Ral GTPases have been implicated as critical drivers of cell growth and metastasis in numerous Ras-driven cancers. Upon association with and activation by Ras·GTP, RalGDS activates the Ral (Ras-like) small GTPases, RalA, and RalB. The Ral GTPases share a panel of effectors including RLIP76 (also called RalBP1), members of the exocyst complex (Sec5 and Exo84), and the transcription factor ZONAB. Our solution structure of the RBD of RLIP76 in complex with RalB revealed that the interaction is mediated by a well-structured coiled-coil domain in which more than 80% of the interactions with Ral are mediated by the C-terminal α2 helix.

The tightest binding sequences, termed HLR (E427H/Q433L/K440R) and SMLR (E427S/L429M/Q433L/K440R), displayed affinities of 5 and 3 nM for RalA, respectively, a vast improvement on the wild-type RBD affinity of around 100 nM. We obtained high-quality crystals for both the RalB/RLIP76 RBD HLR and SMLR mutant complexes, which diffracted to 1.5 Å resolution. ITC revealed that the Q433L mutation was the key driver for improved affinity, resulting in a ∼20 to 30-fold improvement in affinity compared with the wild-type RBD. Crystal structures of the HLR and SMLR mutant RBDs in complex with RalB revealed that this leucine side chain is able to sustain a network of hydrophobic interactions involving Ral and RBD residues. The mutant RBD structures show that the side chain of Leu433 contributes to a hydrophobic network of interactions involving several Ral residues (Ala48, Leu67, Tyr82) and Trp430 of RLIP76. In the wild-type RBD complex, Gln433 points out to the solvent, leaving a space at the edge of the hydrophobic pocket where Trp430 is buried in an interaction known to be essential for the binding affinity. When the Gln is replaced by Leu, the side chain shifts toward the pocket and fills this space. Lys440 forms a hydrogen bond with RalB Asp49 in the wild-type complex and this interaction has been shown to be critical for binding to Ral, as alanine replacement reduced the affinity tenfold. Replacement with arginine in the HLR and SMLR mutants allows this hydrogen bond to be maintained while an additional hydrogen bond with the backbone carbonyl of RalB Ala48 is gained. The replacement of Glu427 with histidine or serine breaks a salt bridge formed with RalB without forming any new interactions and ITC data demonstrated that this substitution did not improve binding to Ral proteins.

>MAANKSKGQSSLALHKVIMVGSGGVGKSALTLQFMYDEFVEDYEPTKADSYRKKVVLDGEEVQIDILDTAGLEDYAAIRDNYFRSGEGFLLVFSITEHESFTATAEFREQILRVKAEEDKIPLLVVGNKSDLEERRQVPVEEARSKAEEWGVQYVETSAKTRANVDKVFFDLMREIRTKKMSENK[2x];>GPLGSETQAGIKEEIRRQEFLLNSLHRDLQGGIKDLSKESRMWEVLRILTALRRKLREA[2x]> MAQQKKTIAVVNATGRQAASLIRVAAAVGHHVRAQVHSLKGLIAEELQAIPNVTLFQGPLLNNVPLMDTLFEGAHLAFINTTSQAGDE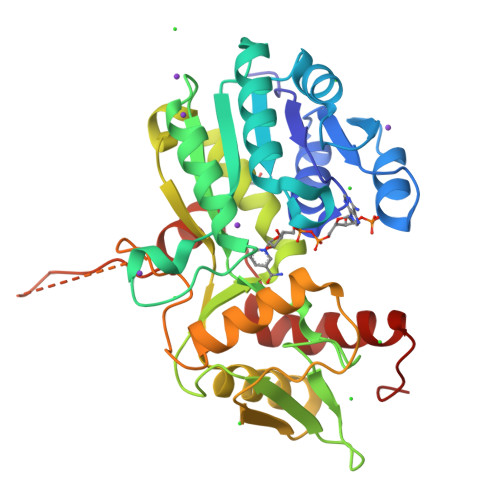IAIGKDLADAAKRAGTIQHYIYSSMPDHSLYGPWPAVPMWAPKFTVENYVRQLGLPSTFVYAGIYNNNFTSLPYPLFQMELMPDGTFEWHAPFDPDIPLPWLDAEHDVGPALLQIFKDGPQKWNGHRIALTFETLSPVQVCAAFSRALNRRVTYVQVPKVEIKVNIPVGYREQLEAIEVVFGEHKAPYFPLPEFSRPAAGSPKGLGPANGKGAGAGMMQGPGGVISQRVTDEARKLWSGWRDMEEYAREVFPIEEEANGLDWML>MGSSHHHHHHSSGRENLYFQGVQHTIARWVDRLREEYADAVAILLKGSYARGDAATWSDIDFDVLVSTQDVEDYRTWIEPVGDRLVHISAAVEWVTGWERDTVDPSSWSYGLPTQETTRLMWAINDETRRRLDRPYKTHPAAEPEVEDTVEALGKIRNAIARGDDLGVYQSAQTVAKLVPTLLIPINPPVTVSHARQAIEAILAFPRVPVGFAADWLTCLGLVEERSARSTAAAAERMVRGVLEMLPTDPDLLGEDIA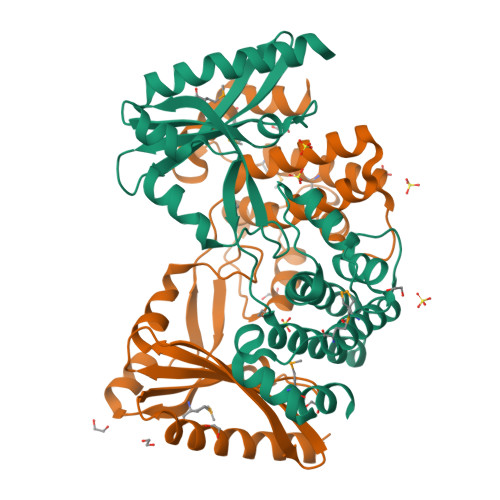RLMNAGLLEKYVQQ[2x]> PPDPQVRCPSVIEFGKYEIHTWYSSPYPQEYSRLPKLYLCEFCLKYMKSRTILQQHMKKCGWFHPPANEIYRKNNISVFEVDGNVSTIYCQNLCLLAKLFLDHKTLYYDVEPFLFYVLTQNDVKGCHLVGYFSKEKHCQQKYNVSCIMILPQYQRKGYGRFLIDFSYLLSKREGQAGSPEKPLSDLGRLSYMAYWKSVILECLYHQNDKQISIKKLSKLTGICPQDITSTLHHLRMLD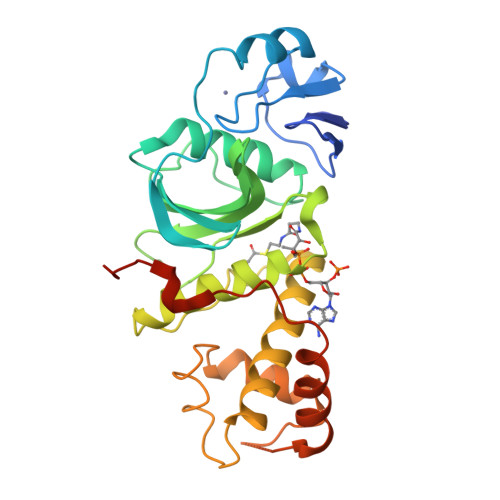FRSDQFVRRRREKLIQDHMAKLQLNLRPVDVDPECLRWTPVIVSNSKKK> MKRQGKRPSKNLKARCSRKALHVNFKDMGWDDWIIAPLEYEAFHCEGLCEFPLASHLEPTNHAVIQTLMNSMDPESTPPTCCVPTRLSPISILFIDSANNVVYKQYEDMVVESC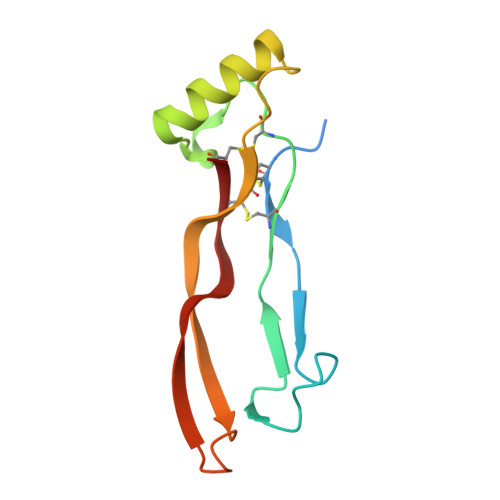GCR>[3x]MRTRSTISTPNGITWYYEQEGTGPDVVLVPDGLGECQMFDSSVSQIAAQGFRVTTFDMPGMSRSAKAPPETYTEVTAQKLASYVISVLDALDIKHATVWGCASGASTVVALLLGYPDRIRNAMCHELPTKLLDHLSNTAVLEDEEISKILANHMLNDVSGGSEAWQAMGDEVHARLHKNYPVWARGYPRTIPPSAPVKDLE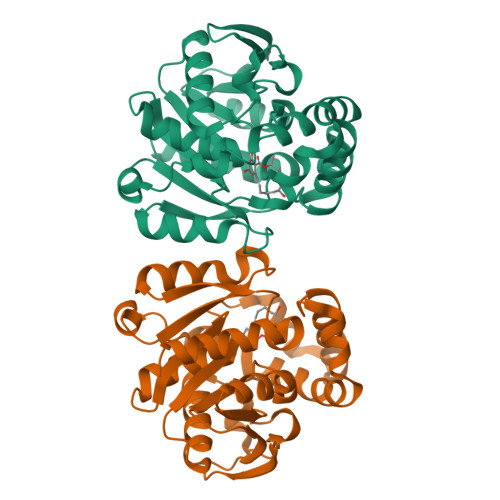ALRGKPLDWTVGAATPTESFFDNIVTATKAGVNIGLLPGMHFPYVSHPDVFAKYVVETTQKHL> MAHHHHHHMASADVVSTWV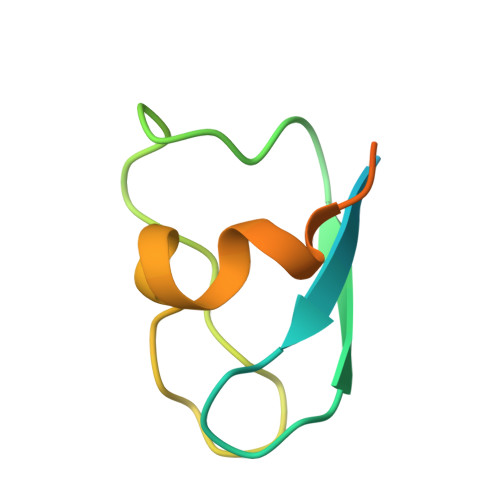CPICMVSNETQGEFTKDTLPTPICINCGVPADYELTKSSINCSNAIDPNANPRNQFG> GAMDGSQGSTDYGDHVVLRYGGTREM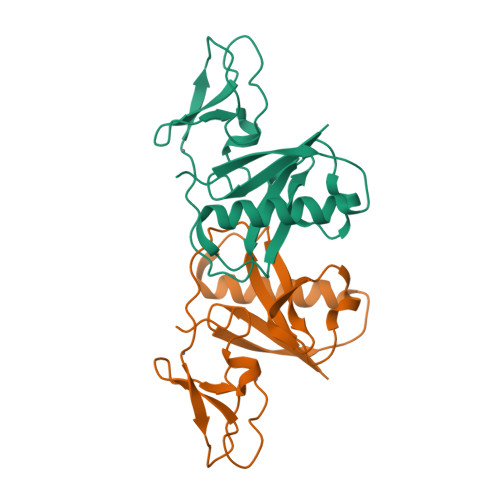VPLIRHEQMLDMLMERARQIVQGFGNLDTRNMYLFRHEYNSPTLLYPITSASQITSGSILEIILVDRTEAAVIPHVVEPESYMRPTFCDFCGEMLTGLMRQGVKCKNCNGNFHKRCSNAARNNCGAP>[4x]GEIEFIESSKDA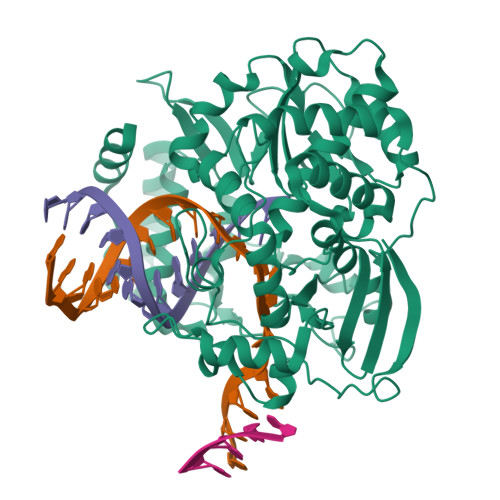GFPVINTPSKTKLEPSVFHQVFEGNKEPAVLRSGDPRLKANFEEAIFSKYIGNVNTHVDEYMLEAVDHYAGQLATLDISTEPMKLEDAVYGTEGLEALDLTTSAGYPYVALGIKKRDILSKKTKDLTKLKECMDKYGLNLPMVTYVKDELRSIEKVAKGKSRLIEASSLNDSVAMRQTFGNLYKTFHLNPGVVTGSAVGCDPDLFWSKIPVMLDGHLIAFDYSGYDASLSPVWFACLKMILEKLGYTHKETNYIDYLCNSHHLYRDKHYFVRGGMPSGCSGTSIFNSMINNIIIRTLMLKVYKGIDLDQFRMIAYGDDVIASYPWPIDASLLAEAGKGYGLIMTPADKGECFNEVTWTNVTFLKRYFRADEQYPFLVHPVMPMKDIHESIRWTKDPKNTQDHVRSLCLLAWHNGEHEYEEFIRKIRSVPVGRCLTLPAFSTLRRKWLDSFGSSSHHHHHH8-butyl-1-methyl-7-(2-methylphenyl)-1H-imidazo[2,1-f]purine-2,4(3H,8H)-dione 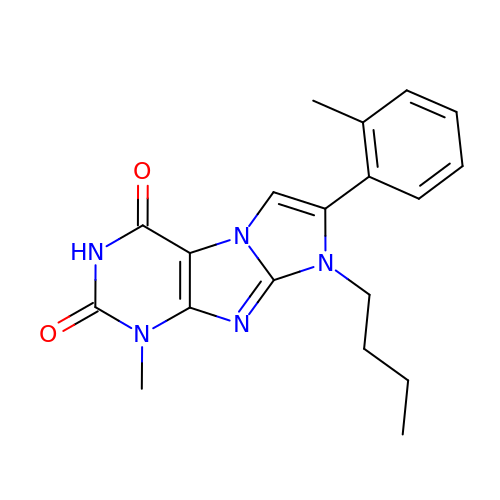| C19 H21 N5 O2 | KCEWOOVCWCPFCY-UHFFFAOYSA-N>MPDELKPHFANVQAHYDLSDDFFRLFLDPTQTYSCAYFERDDMTLQEAQIAKIDLALGKLGLQPGMTLLDVGCGWGATMMRAVEKYDVNVVGLTLSKNQANHVQQLVANSENLRSKRVLLAGWEQFDEPVDRIVSIGAFEHF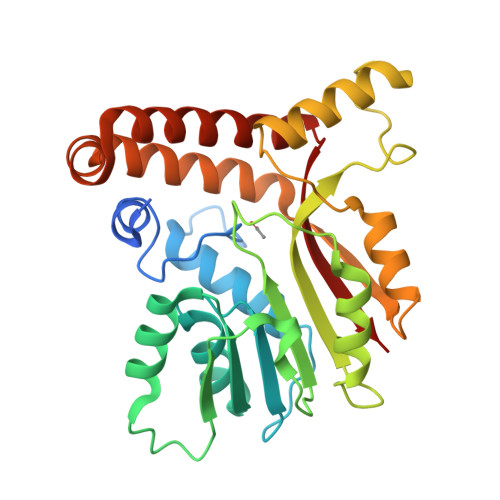GHERYDAFFSLAHRLLPADGVMLLHTITGLHPKEIHERGLPMSFTFARFLKFIVTEIFPGGRLPSIPMVQECASANGFTVTRVQSLQPHYAKTLDLWSAALQANKGQAIALQSEEVYERYMKYLTGCAEMFRIGYIDVNQFTCQK[2x]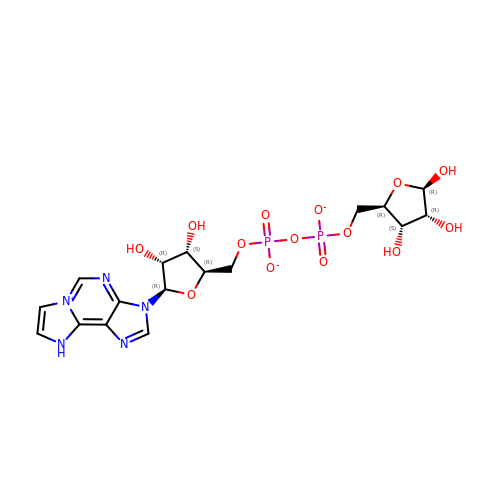[[(2R,3S,4R,5R)-3,4-dihydroxy-5-(9H-imidazo[2,1-f]purin-6-ium-3-yl)oxolan-2-yl]methoxy-oxidanidyl-phosphoryl] [(2R,3S,4R,5R)-3,4-dihydroxy-5-oxidanidyl-oxolan-2-yl]methyl phosphate | C17 H22 N5 O14 P2 | YOABXPSQFWZTMU-QJWJOKBXSA-M>[2x]MVQPFAAQVASLADRYEESFDIGAAVEPHQLNGRQGKVLKHHYNSIVAENAMKPISLQPEEGVFTWDGADAIVEFARKNNMNLRFHTLVWHNQVPDWFFLDEEGNPMVEETNEAKRQANKELLLERLETHIKTVVERYKDDVTAWDVVNEVVDDGTPNERGLRESVWYQITGDEYIRVAFETARKYAGEDAKLFINDYNTEVTPKRDHLYNLVQDLLADGVPI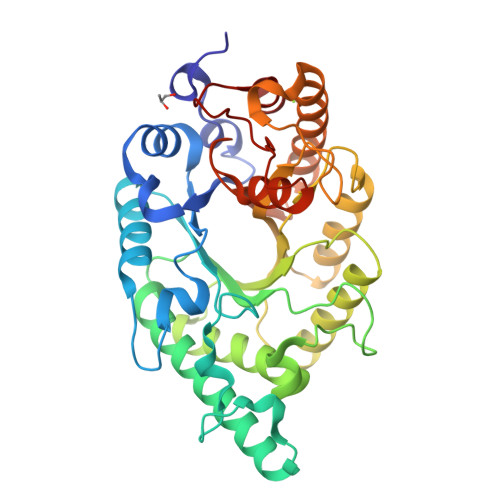DGVGHQAHIQIDWPTIDEIRTSMEMFAGLGLDNQVTELDVSLYGWPPRPAFPTYDAIPQERFQAQADRYNQLFELYEELDADLSSVTFWGIADNHTWLDDRAREYNDGVGKDAPFVFDPNYRVKPAFWRIID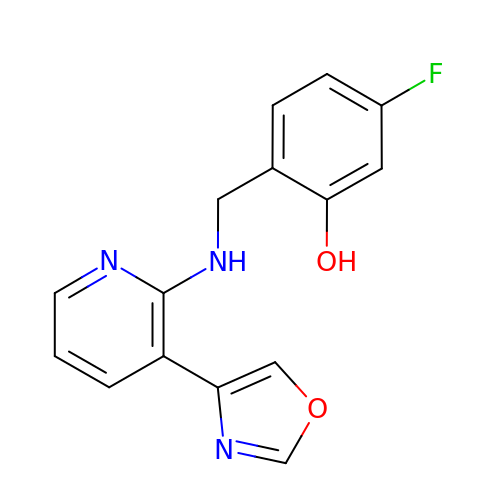5-fluoro-2-({[(3M)-3-(1,3-oxazol-4-yl)pyridin-2-yl]amino}methyl)phenol | C15 H12 F N3 O2 | AIPASLMZJHFYBT-UHFFFAOYSA-N>[2x]KKYFMSSVRRMPLNRAKALCSELQGTVATP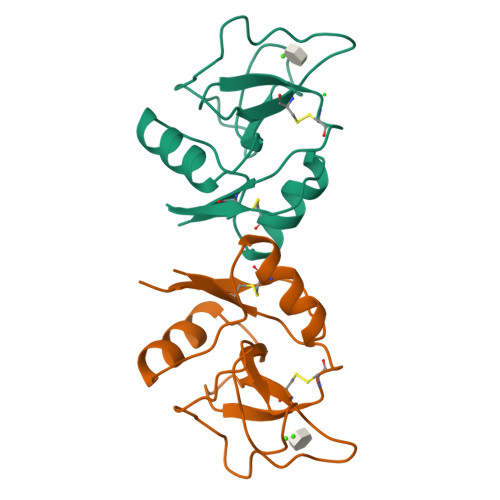RNAEENRAIQNVAKDVAFLGITDQRTENVFEDLTGNRVRYTNWNEGEPNNVGSGENCVVLLTNGKWNDVPCSDSFLVVCEFSD2-chloro-9-(3-(2,2-difluoroethoxy)-5-isopropoxybenzyl)-9H-purin-6-amine | C17 H18 Cl F2 N5 O2 | 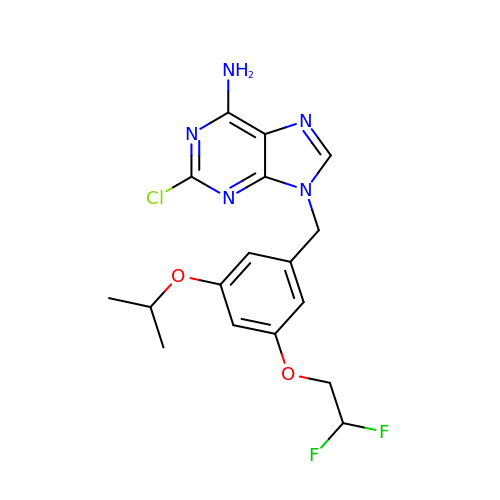VOYIVHUUVWJRDM-UHFFFAOYSA-N> AFAGILADADCAAAVKACEAADSFSYKAFFAKCGLSGKSADDIKKAFVFIDQDKSGFIEEDELK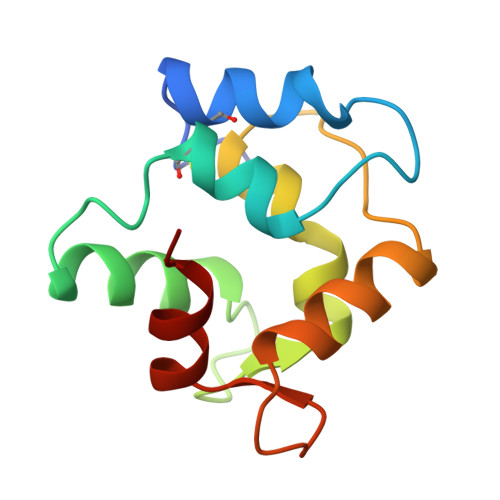LFLQVFKAGARALTDAETKAFLKAGDSDGDGAIGVEEWVALVKA> M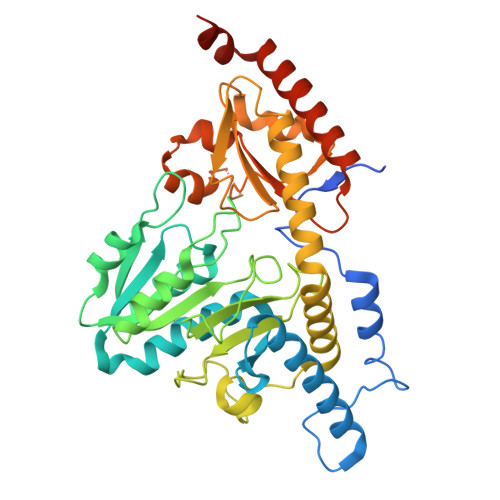GSSHHHHHHGSMYGVYRAMKLPIYLDYSATTPVDPRVAEKMMQFMTMDGTFGNPASRSHRFGWQAEEAVDIARNQIADLVGADPREIVFTSGATESDNLAIKGAANFYQKKGKHIITSKTEHKAVLDTCRQLEREGFEVTYLAPQRNGIIDLKELEAAMRDDTILVSIMHVNNEIGVVQDIAAIGEMCRARGIIYHVDATQSVGKLPIDLSQLKVDLMSFSGHKIYGPKGIGALYVRRKPRVRIEAQMHGGGHERGMRSGTLPVHQIVGMGEAYRIAKEEMATEMERLRGLRNRLWNGIKDIEEVYLNGDLEHGAPNILNVSFNYVEGESLIMALKDLAVSSGSACTSASLEPSYVLRALGLNDELAHSSIRFSLGRFTTEEEIDYTIELVRKSIGRLRDLSPLWEMYKQGVDLNSIEWAHH5,6-dihydroorotidine 5'-monophosphate | C10 H15 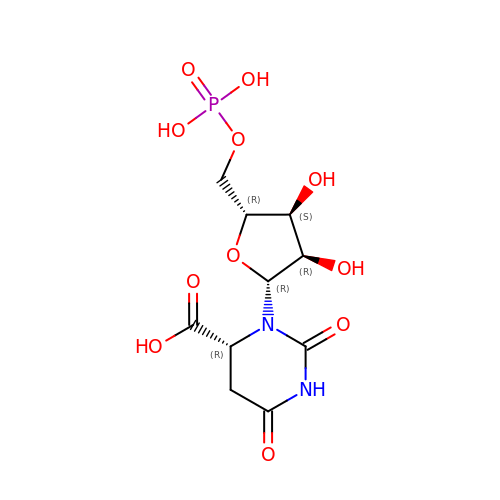N2 O11 P | ZVESSEXVBFSYOC-NFTAXOAUSA-N>[2x]GAMALYEFVGLLDAHGNVLEVNQVALEGGGITLEEIRGKPFWKARWWQISKKTEATQKRLVETASSGEFVRCDVEILGKSGGREVI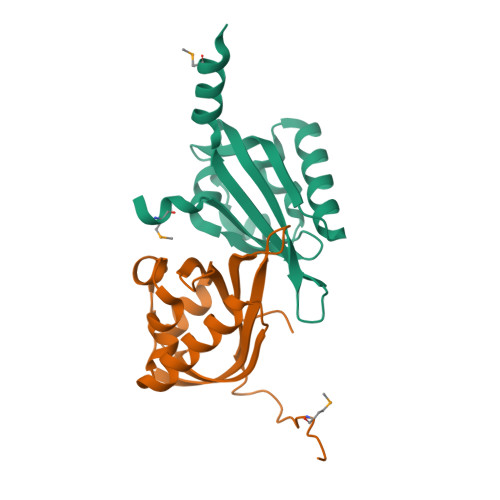AVDFSLLPICNEEGSIVYLLAEGRNITDKKKAEAMLALKNQELE> VCNRLEQILVKTQWAQSYGEAENRAAFSRDLFSELFNIQGSSRALFSGVGVDDMNSAAFTAHCLRVTGALNRLISQLDQQATINADLAHLAGQHASRNLDASNFAAMGQAVMSVVPTHLDCFNQHAWGECYERIASGISG;> DCTSLNRLLVKRQWAEAYGEGTNRELLGNRIWEDLFANMPDARGLFSRVNGNDIDSSEFQAHSLRVLGGLDMCVASLDDVPVLNALLARLNSQHDSRGIPAAGYPAFVASAISAVRATVGARSFDNDAWNSCMNQIVSGISG;> SSCCSSEDRANVMHNWDAAWSAAYSDRRVALAQAVFASLFSRDAAAQGLFSGVSADNPDS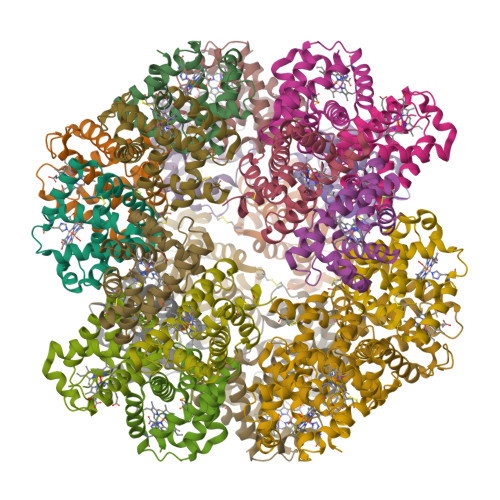ADFRAHCVRVVNGLDVAINMLNDPAVLNEQLAHLSAQHQARAGVAAAHFDVMAEAFAEVMPQVSSCFSSDSWNRCFARIANGISAGL;> ECCSRGDAEVVISEWDQVFNAAMAGSSESAVGVAIFDAFFASSGVSPSMFPGGGDSNNPEFLAQVSRVVSGADIAINSLTNRATCDSLLSHLNAQHRAISGVTGAAVTHLSQAISSVVAQVLPSAHIDAWEYCMAYIAAGIGAGL>[2x]MVRNLVIDITKKPTQNIPPTNEIIEEAITELNVDELLDRLFEKDESGEVITPSRIAKMLEEKAFEIYKEYEKQVREAYLSAGYSREKLEQSFQQARFSRGGKAFEIIFTKLLNKFGIRYEHDRVIKIYDYITEGEKPAFIIPSVRTFLNDPSSAILITVKRKVRERWREAVGEAQILRNKFGDEINFWFVGFDEEFTIYSAIAMLDNGIDRVY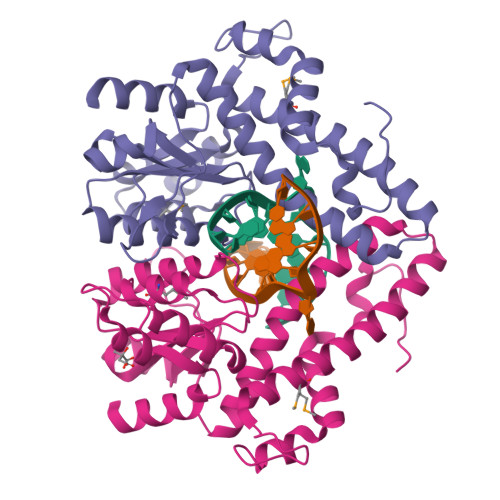VIDGRYDSLIEEIKRISDPNFNEDKYIQKIRRFSDIFDDIIQFLNKHGNKKRGKQLTLV>[2x]MGSDKIHHHHHHENLYFQGMNDTIARYFDAFNAGDTDGMLACLSEDVAHHVNEGNIRVGKEKFAAFCAHMSHCYKEELTDM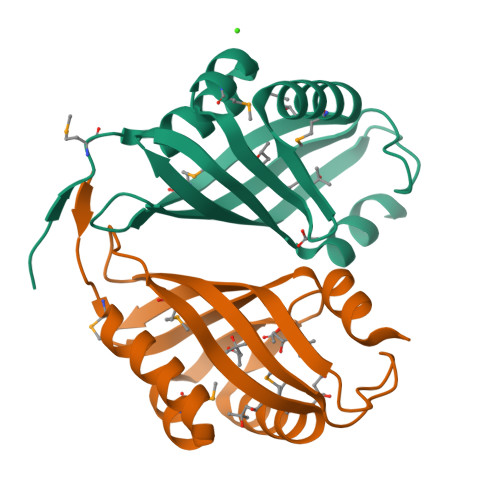VIFATPDATRAAAEYTVNGTYLATDEGLPEARQQSYKLPAGSFFDLRDGLITRVTTYYNLSDWIKQVSA>[2x]MERYESLFAQLKERKEGAFVPFVTLGDPGIEQSLKIIDTLIEAGADALELGIPFSDPLADGPTIQNATLRAFAAGVTPAQCFE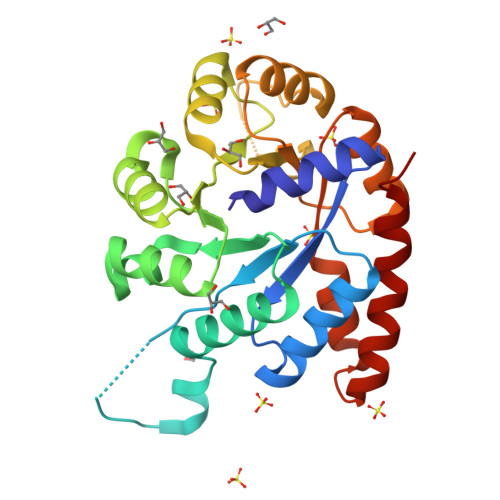MLALIRQKHPTIPIGLLMYANLVFNKGIDEFYAQCEKVGVDSVLVADVPVEESAPFRQAALRHNVAPIFICPPNADDDLLRQIASYGRGYTYLLSRAGVTGAENRAALPLNHLVAKLKEYNAAPPLQGFGISAPDQVKAAIDAGAAGAISGSAIVKIIEQHINEPEKMLAALKVFVQPMKAATRS> GPHMAEEAYKQQIKEDNIGNQLLRK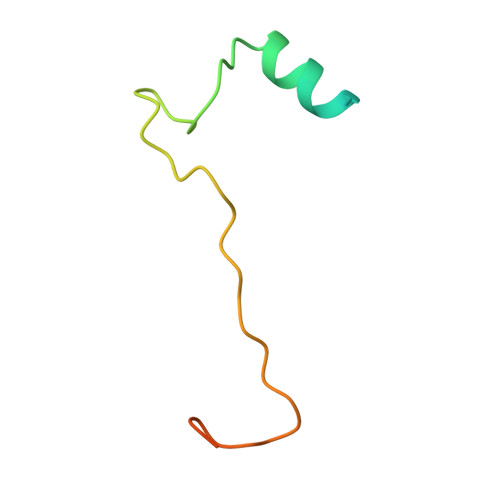MGWTGGGLGKSGEGIREPISVKEQHKREGLGLDVERVNKIAK>[2x]HHHHHHHHGGLVPRGSHGGSMTDRLKGKVAIVTGGTLGIGLAIADKFVEEGAKVVITGRHADVGEKAAKSIGGTDVIRFVQHDASDEAGWTKLFDTTEEAFGPVTTVVNNAGIAVSKSVEDTTTEEWRKLLSVNLDGVFFGTRLGIQRMKNKGLGASIINMSSIEGFVGDPTLGAYNAS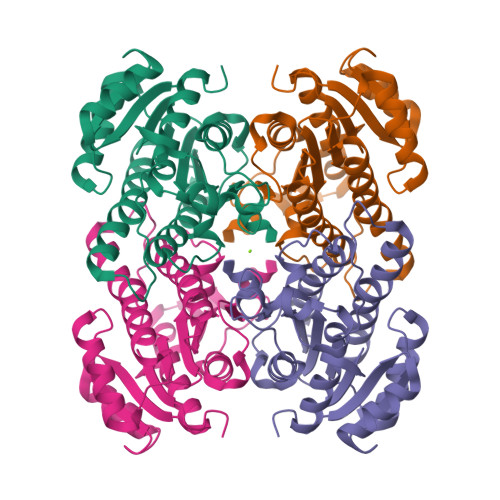KGAVRIMSKSAALDCALKDYDVRVNTVHPGYIKTPLVDDLEGAEEMMSQRTKTPMGHIGEPNDIAWICVYLASDESKFATGAEFVVDGGYTAQ> FQSNAMKHCPITYEKISDQENYSQRGLHLLSPQLKNLSPLDLSADEQRQEAIARVGKMSVQGVQKKLSAKLKIKEGCFEIVDQYGQYILKPQSDIYPELPENEAITMTLAKTIGLEVPVHGLVYSKDNSLTYFIKRFDRIGHNKKLALEDFAQLSGEDRHTKYKSSMEKVIAVIEQFCTFPKIEFVKLFKLTLFNFLVGNEDMHLKNFSLITKDRKISISPAYDLLNSTIAQKNTKEELALPLKGKKNNLTKSDFLKYFAIEKLGLNQNVIDGIVQEFHQVIPKWQELIGFSFLSQEMQEKYLELLEQRCKRLNFFD;> MRKAYVSVSGIKAGILEELQGGTYQFTYFEDYHGAPVSLTMPLKNKVYDFDVFPPFFEGLLPEGIMLEALLRKYKIDKNDYFGQLILVGQDVVGAVTIEEIR

Here, we perform structural and biochemical characterization of the Legionella pneumophila effector Lpg2370, demonstrating that it is a Ser/Thr kinase. Together with two upstream genes, lpg2370 constitutes the tripartite HipBST TA. Notably, the toxin Lpg2370 (HipTLp) and the antitoxin Lpg2369 (HipSLp) correspond to the C-terminus and N-terminus of HipA from HipBA TA, respectively. Structural analysis reveals that HipSLp binding induces a loop-to-helix shift in the P-loop of HipTLp, leading to the blockage of ATP binding and inhibition of the kinase activity.

The crystal structure of the SeMet-labeled HipTLp–HipSLp complex was determined and refined at 1.89 Å resolution. In the structure of HipTLp–HipSLp complex, a copy of HipTLp and HipSLp each were observed per crystal asymmetric unit. Residues belonging to helices α1 and α2 of HipTLp were not visible in the electron density map, whereas the density of the remaining residues was unambiguous. All 102 residues of HipSLp were successfully built into the model, showing that HipSLp is a small single-domain protein composed of five β-strands and three α-helices. In the structure of HipTLp–HipSLp complex, three α-helices of HipSLp form a helix bundle that sits above the cleft formed by the β-sheet in the N-terminal lobe of HipTLp, whereas the β-strands form a flank region in HipSLp. HipSLp binds the toxin HipTLp via hydrogen bonding in three main interacting regions, which constitute more than 1100 Å2 of total buried surface area. The intermolecular interactions are mainly formed between helices α1, α2 and α1–α2 loop of HipSLp and helix α3 and strand β5 of HipTLp. The HipTLp mutants D133A, R134A, and E144A completely lost their ability to bind HipSLp and the mutants R154A, K157A, K201A exhibited severely reduced HipSLp binding, suggesting that these residues form key interactions with HipSLp. Notably, Ser54 of HipTLp is phosphorylated in the structure of apo pHipTLp but not in the HipTLp–HipSLp complex (please note that HipTLp–HipSLp was co-expressed in E. coli BL21). Moreover, structural comparison suggests that the P-loop of HipTLp, which encircles ATP and is critical for catalytic activities in typical Ser/Thr kinases, underwent a conformational change from loop to helix upon HipSLp binding.(S)-1-(2-AMINO-2-CARBOXYETHYL)-3-(2-CARBOXYBENZYL)PYRIMIDINE-2,4-DIONE 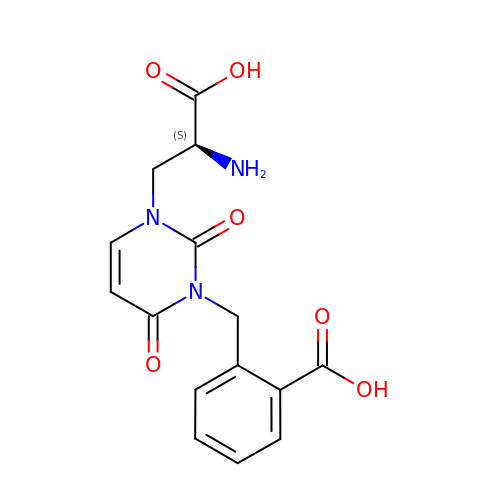| C15 H15 N3 O6 | UUIYULWYHDSXHL-NSHDSACASA-N>[2x]SNAVNLFGQKDRGNHVSGVDRG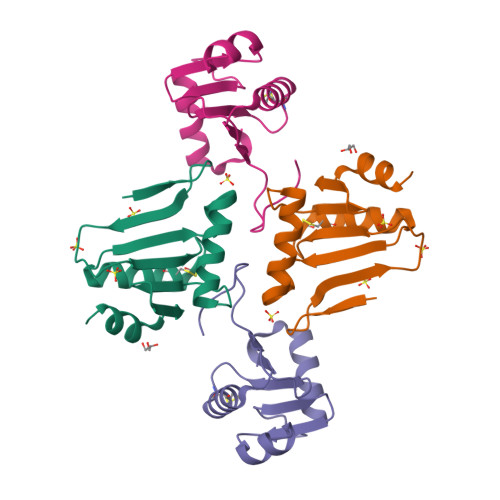KVIMYGLSTCVWCKKTKKLLTDLGVDFDYVYVDRLEGKEEEEAVEEVRRFNPSVSFPTTIINDEKAIVGFKEKEIRESLGF>[4x]MGSDKIHHHHHHENLYFQGMGTDKFNNIKIDKYENLINVLKTGDIFLCSGNYLVSKLIKKVSESMFSHTGIIVKWGEHTLIMESVEDDGVRIVPLEHYIKNYENSNNRYNGSLFIARHELLQNVNDDSEMIRNLIKVGFSLLNSGYDKNEIAQIVARIGLGIGRHEDNNEYICSEFVNECFKKIGVEFLTDSEGFIFPEHIAADHHVLPIAQIE

NlpC/P60 superfamily proteins are ubiquitous papain-like cysteine peptidases or other functionally related enzymes. To provide insights into the function of these biologically important proteins, as well as PPNEs in general, we report the crystal structure of BcPPNE and a comparative structural analysis to other related PPNEs. Our results suggest that BcPPNE and YiiX are likely amidases with specificity for the amide bond between a lipid and an amino acid (or peptide).

The data were indexed in space group P65 and the structure was determined to a resolution of 2.5 Å with four molecules per asymmetric unit (asu) using the SAD method (Rcryst = 19.2/Rfree = 21.9). The final structure of BcPPNE contains four monomers (A, residues 2–195; B, residues −3–195; C residues −4–195; and D, residues 0–195, where residues upstream of 1 are a part of the purification tag), with a lysine bound in each active site, nine chloride ions and 41 waters. Each monomer consists of a layered α/β fold with a central, 6-stranded, antiparallel β-sheet (β1–β6), which is protected by helices on either side (αA and αC on one side, αD, αF and αG the other). Extra, unaccounted-for, electron density was identified at the entrance to the active site of each BcPPNE monomer and was modeled as an L-lysine based on shape and electrostatic complementarity. The lysine occupies the S1′ subsite and forms a hydrogen-bond network with several conserved protein residues (Ser48, His49, Glu67, Asp68, Tyr83, and Tyr90). One striking feature of the active site pocket of BcPPNE is that the tight fit of the binding cavity around the bound lysine at S1′ renders the catalytic cysteine inaccessible to solvent, suggesting induced-fit binding. Side chains of Glu67 and Asp68 interact with the free main-chain amine group and the side-chain Nζ of the lysine, respectively. In this conformation, Glu67 occupies the position expected for Tyr127, based on comparison with other NlpC/P60 structures. As a result, the bound lysine seems to have induced the rearrangement of a short loop (residues 66–69), containing Glu67 and Asp68, which, in turn has displaced Tyr127 from its (expected) original location. Thus, we conclude that the ternary complex of BcPPNE may represent a “closed” (or inhibited) conformation of the enzyme.> MSTFEDADTEETVTCLQMTIYHPGQQSGIFKSIRFSSKEKFPSIEVVKFGRNS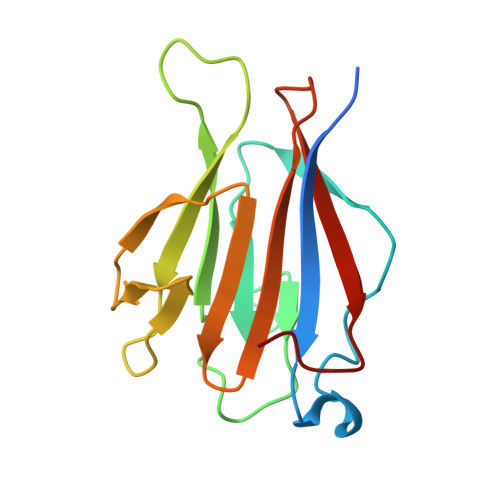NMCQYTFQDKQVSRIQFVLQPFKQFNSSVLSFEIKNMSKKTSLMVDNQELGYLNKMDLPYKCMLRFGEYQFLLQKEDGESVESFETQFIMSSRPLLQ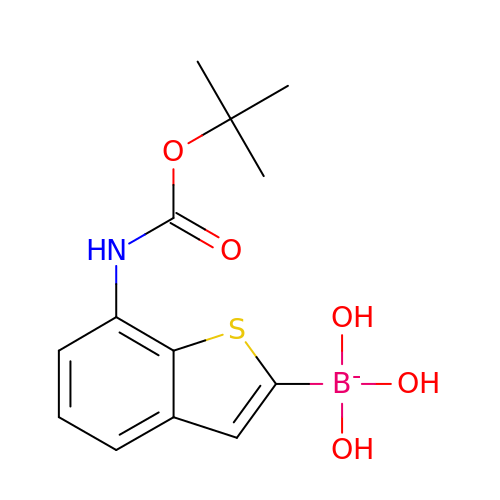[7-[(2-methylpropan-2-yl)oxycarbonylamino]-1-benzothiophen-2-yl]-tris(oxidanyl)boranuide | C13 H17 B N O5 S | WAKYUFAFDTZJQR-UHFFFAOYSA-N> MGNTSSERAALERHGGHKTPRRDSSGGTKDGDRPKILMDSPEDADLFHSEEIKAPEKEEFLAWQHDLEVNDKAPAQARPTV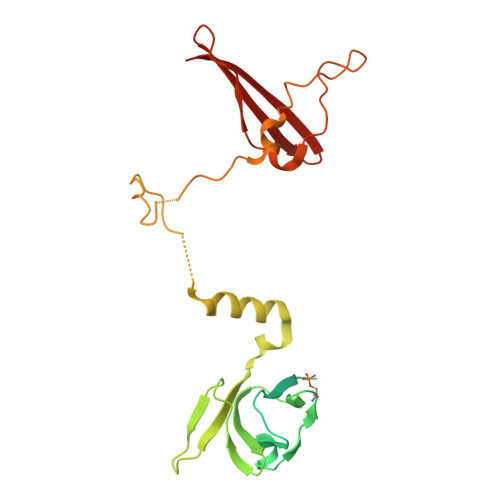FRWTGGGKEVYLSGSFNNWSKLPLTRSHNNFVAILDLPEGEHQYKFFVDGQWTHDPSEPIVTSQLGTVNNIIQVKKTDFEVFDALMVDSQKCSDVSELSSSPPGPYHQEPYVCKPEERFRAPPILPPHLLQVILNKDTGISCDPALLPEPNHVMLNHLYALSIKDGVMVLSATHRYKKKYVTTLLYKPI> MRAPIPEPKPGDLIEIFRPFYRHWAIYVGDGYVVHLAPPSEVAGAGAASVMSALTDKAIVKKELLYDVAGSDKYQVNNKHDDKYSPLPCSKIIQRAEELVGQEVLYKLTSENCEHFVNELRYGVAR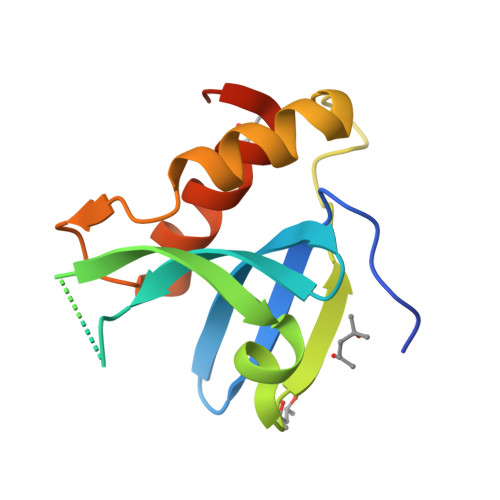SDQVRD> ETPPRFTRTPVDQTGVSGGVASFICQATGDPRPKIVWNKKGKKVSNQRFEVIEFDDG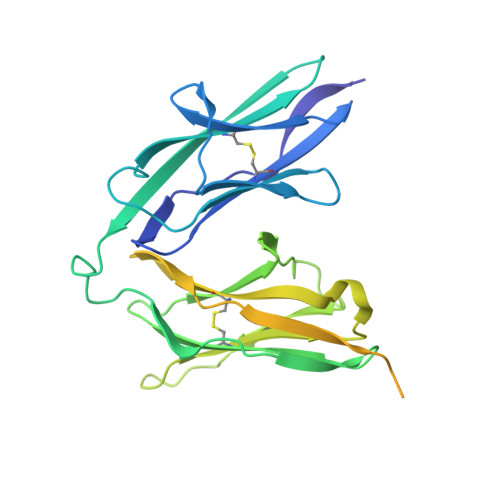SGSVLRIQPLRTPRDEAIYECVASNNVGEISVSTRLTVLREDQIPRGFPTIDMGPQLKVVERTRTATMLCAASGNPDPEITWFKDFLPVDTSNNNGRIKQLRSESIGGTPIRGALQIEQSEESDQGKYECVATNSAGTRYSAPANLYVRELREVRRVPPRFSIPPTNHEIMPGGSVNITCVAVGSPMPYVKWMLGAEDLTPEDDMPIGRNVLELNDVRQSANYTCVAMSTLGVIEAIAQITKHHHHHH> ASPSSELRRALEANEFIPYYQPLSPGQGGRWIGVEVLMRWRHPREGLIRPDLFIPFAERSGLIVPMTRALMRQVAEDLGGHAGKLEPGFHIGFNISATHCHELALVDDCRELLAAFPPGHITLVLELTERELIESSEVTDRLFDELHALGVKIAIDDFGTGHSSLAYLRKFQVDCLKIDQSFVARIGIDTLSGHILDSIVELSAKLDLDIVAEGVETPEQRDYLAARGVDYLQGYLIGRPMPLESLLSSLTVQEQQ

DGC domains containing the signature GGDEF motif synthesise c-di-GMP from two GTP molecules while EAL1516 and HD-GYP171819 domain-containing PDEs are responsible for the hydrolysis of c-di-GMP to 5′-phosphoguanylyl-(3′-5′)-guanosine (pGpG). Hydrolysis of c-di-GMP by EAL domains has been shown to require the presence of divalent ions, either Mg2+ or Mn2+, with the most efficient reactions occurring at alkaline pH2933. Here we report as yet structurally uncharacterised EAL domains from the core genome of Pseudomonas aeruginosa, PA1727 (MucR) and PA3825.

We determined the PDE domain structures of MucREAL and PA3825EAL in complex with c-di-GMP/Mg2+. The structure of PA3825EAL in complex with c-di-GMP/Mg2+ shows a different dimer interface to MucR, named here as the “closed dimer”. The Mg2+ and Ca2+ complexes show metals in the catalytic centre, annotated as M1 and M2, coordinating the phosphate group of the scissile phosphodiester in c-di-GMP. In both cases, the metal is coordinated in an octahedral geometry by Glu39, Asn98, Asp130, Asp160, a non-bridging oxygen from the scissile phosphate (P1) of c-di-GMP and a putative in-line attacking water molecule. Significant differences are seen in the positioning of the Asp160 side chain between metal bound complexes, with the second oxygen of Asp160 contacting a peptide nitrogen atom with Mg2+ bound; while the Ca2+ bound complex shows Asp160 bridging between the M1 and M2 metals. The M2 metal shows octahedral coordination for Mg2+ but trigonal bipyramidal coordination geometry for Ca2+. Mg2+ is coordinated by Asp161, Asp183, a non-bridging phosphate (P1) oxygen and two waters. The β5-α5 loop of PA3825EAL, residues 160–170, undergo significant changes between Mg2+-c-di-GMP bound and metal-free-apo states. The β5-α5 loop moves towards the active site and contributes to the formation of metal binding sites via two highly conserved Asp residues (Asp160–161). The restructuring of the β5-α5 loop and the functional role in metal coordination is thus conserved across different dimer interfaces.>[2x]MMQFTMSGTMLRFDETTLRFSFSRDGATWSGCDGIEPQLTREDRSFSFAGAATVTHERIETGTGVGVRSVF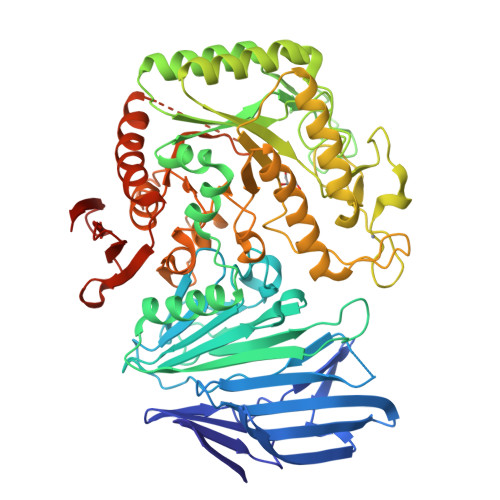AGFAGADYAFETYIWIERSSGDVLCEWVPLRECGAEPRIDRVLWPAPLSFDRADAHDVTLITHEQGVMIPNSWPTEVGTDAVSFGGRFETAGGYMPWFAQLRSDGHAYIAICETPWNAGYDIDHPAGGPYTHVGMWFEPSLGRMDYRRVVRYRLLDHADHTAICKTYRAYVNERGRLRTLAEKAARNPSVRDLLGRSWVAVGIKTNVQPDSSFYDPAQPGKNDSLVTFAQRERQMRTLHEMGAGRLYLALAGWAQPGYDNGHPDYLPACREAGGWKGMKSLIDACHEQGDLFGTADQYRDYYFAARTFDPRNAIRLADGTMPEHAMWAGGRQTYLCAELAPDYVRRNFSEIATHGIVLDCAYLDVFTCNEGDECSHPEHRMTRRECYERRAECFEYLLAHGILTSSEEVSDWAVPSLVFCHYAPYDFQMRSPDAPRHGIPVPLYNLVYHDCVIQPWMMDRVAGGDDYMLYALLNGGAPYLIRDAAYAGMDGDMNAALRARTENDIERCAVVAGLHRRVGMQELVRHDLVGGDPLVQRSVFADGTAVTCDFHAQTYEVAANGSHHHHHHH> MAMAQELTAMSAWVNQDGSTLYINSINAQGELTGSYINRAAGAACQNSPYPVNGWVFGTAISFSTKWLNSVESCNSITSWSGFYINTGGQGKISTLWQLV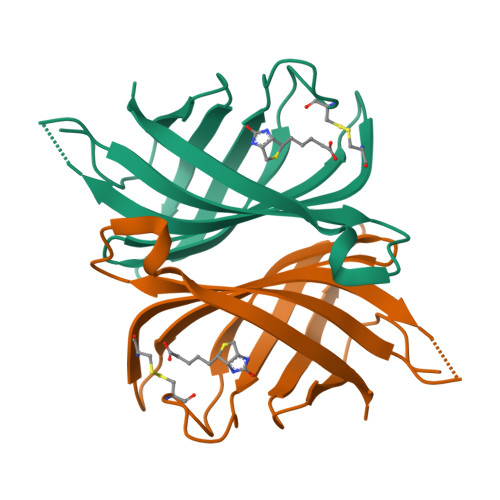VNGSSSPSQILKGQDVFSQTSA> MRVKHAVVLLMLISPLSWAGTMTFQFRNPNFGGNPNNGAFLLNSAQAQNSYKDPSYNDDFGIETPSALDNFTQAIQSQILGGLLSNINTGKPGRMVTNDYIVDIANRDGQLQ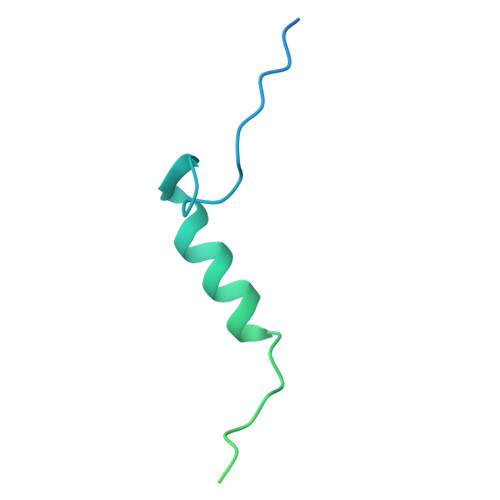LNVTDRKTGQTSTIQVSGLQNNSTDF> MAFSVLNWDQVSRLHEVLTEVVPIHGRGNFPTLEITLKDIVQTVRSRLEEAGIKVHDVRLNGSAAGHVLVKDNGLGCKDLDLIFHVALPTEAEFQLVRDVVLCSLLNFLPEGVNKLKISPVTLKEAYVQKLVKVCTDTDRWSLISLSNKNGKNVELKFVDSIRRQFEFSVDSFQIILDSLLFFYDCSNNPISEHFHPTVIGESMYGDFEEAFDHLQNRLIATKNPEEIRGGGLLKYSNLLVRDFRPTDQEEIKTLERYMCSRFFIDFPDILEQQRKLETYLQNHFAEEERSKYDYLMILRRVVNESTVCLMGHERRQTLNLISLLALRVLAEQNIIPSATNVTCYYQ;> RTLRSITSPLVAHRLKPIRQKTKKAVVSILDSEEVCVELVKEYASQEYVKEVLQISSDGNTITIYYPNGGRGFPLADRPPSPTDNISRYSFDNLPEKYW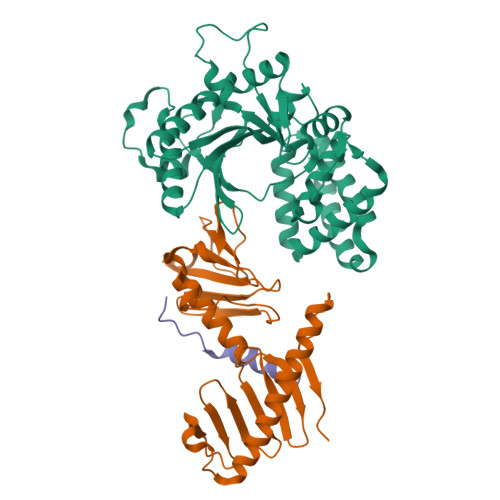RKYQYASRFVQLVRSKSPKITYFTRYAKCILMENSPGADFEVWFYDGVKIHKTEDFIQVIEKTGKSYTLKSESEVNSLKEEIKMYMDHANEGHRICLALESIISEEERKTRSAPFFPIIIGRKP;> IDDEMFYDDHLEAYFEQLAIPG> GPGGDPHMMFGKKKNNGGSSTARYSAGNKYNTLSNNYALSAQQLLNASKIDDIDSMMGFERYVPPQYNGRFDAKDIDQIPGRVGWLTNMHATLVSQETLSSGSNGGGNSNDGERVTTNQGISGVDFYFLDEEGGSFKSTVVYDPYFFIACNDESRVNDVEELVKKYLESCLKSLQIIRKEDLTMDNHLLGLQKTLIKLSFVNSNQLFEARKLLRPILQDNANNNVQRNIYNVAANGSEKVDAKHLIEDIREYDVPYHVRVSIDKDIRVGKWYKVTQQGFIEDTRKIAFADPVVMAFDIETTKPPLKFPDSAVDQIMMISYMIDGEGFLITNREIISEDIEDFEYTPKPEYPGFFTIFNENDEVALLQRFFEHIRDVRPTVISTFNGDFFDWPFIHNRSKIHGLDMFDEIGFAPDAEGEYKSSYCSHMDCFRWVKRDSYLPQGSQGLKAVTQSKLGYNPIELDPELMTPYAFEKPQHLSEYSVSDAVATYYLYMKYVHPFIFSLCTIIPLNPDETLRKGTGTLCEMLLMVQAYQHNILLPNKHTDPIERFYDGHLLESETYVGGHVESLEAGVFRSDLKNEFKIDPSAIDELLQELPEALKFSVEVENKSSVDKVTNFEEIKNQITQKLLELKENNIRNELPLIYHVDVASMYPNIMTTNRLQPDSIKAERDCASCDFNRPGKTCARKLKWAWRGEFFPSKMDEYNMIKRALQNETFPNKNKFSKKKVLTFDELSYADQVIHIKKRLTEYSRKVYHRVKVSEIVEREAIVCQRENPFYVDTVKSFRDRRYEFKGLAKTWKGNLSKIDPSDKHARDEAKKMIVLYDSLQLAHKVILNSFYGYVMRKGSRWYSMEMAGITCLTGATIIQMARALVERVGRPLELDTDGIWCILPKSFPETYFFTLENGKKLYLSYPCSMLNYRVHQKFTNHQYQELKDPLNYIYETHSENTIFFEVDGPYKAMILPSSKEEGKGIKKRYAVFNEDGSLAELKGFELKRRGELQLIKNFQSDIFKVFLEGDTLEGCYSAVASVCNRWLDVLDSHGLMLEDEDLVSLICENRSMSKTLKEYEGQKSTSITTARRLGDFLGEDMVKDKGLQCKYIISSKPFNAPVTERAIPVAIFSADIPIKRSFLRRWTLDPSLEDLDIRTIIDWGYYRERLGSAIQKIITIPAALQGVSNPVPRVEHPDWLKRKIATK

The bulk of DNA synthesis in eukaryotes is carried out by three polymerases: Pols α, δ, and ε. Polε is believed to be the leading strand polymerase and, like Polδ, achieves fidelity via both accurate DNA polymerization and 3′→5′ proofreading exonuclease (Exo) activities. Pols α, δ, and ε belong to the B-family of DNA polymerases. As in the Pol2T:A structure, the Pol2G:C catalytic core surrounds the template-primer with the palm, fingers, thumb and exonuclease domains.

We present here a crystal structure of yeast Pol2 catalytic domain that differs from the Pol2T:A structure in containing a slightly different protein construct (residues 1–1187 versus 1–1228), a different template-primer, a different incoming nucleotide (dCTP versus dATP), a different nascent base pair (G:C versus T:A), and different metals (Ca2+ versus Mg2+). Also, the protein construct we used contains wild-type residues in the exonuclease domain, as opposed to mutations in the Pol2T:A structure (D290A/E292A) which renders it exonuclease deficient. We crystallized the Pol2 catalytic core (residues 1–1187) in ternary complex with a 12-nt/16-nt primer/template presenting G as the templating base, and with dCTP as the incoming nucleotide. To prevent degradation of the DNA by the Pol2 exonuclease activity, we prepared the protein-DNA complex in the presence of Ca2+ (rather than Mg2+). The refined model of Pol2G:C consists of residues 1–1187 (with missing segments 1–29, 215–219, 225–231, 665–677) of Pol2, nucleotides 1–15 of the template, nucleotides 2–12 of the primer, incoming dCTP, 4 Ca2+ ions, 1 Na+ ion, 147 solvent molecules, and 1 molecule of ethylene glycol. Most of the contacts to the nascent G:C base pair occur from atop (Asn828 and Ser829) or from the minor groove side (Tyr 645, Tyr831, and Gly832). Tyr431 lies in a loop (residues 430–439) of the exonuclease domain and approaches the incoming dCTP from the major groove side with its hydroxyl group located ∼4.0 Å from the dCTP N4 atom. The structure reveals Ca2+ ions at positions A and B in the polymerase active site. By contrast, we observe Ca2+ at site B, coordinated by residue Asp290. Surprisingly, this motif is partially disordered in both the Pol2G:C and Pol2T:A structures.> HTLPANEFRCLTPEDAAGVFEIEREAFISVSGNCPLNLDEVQHFLTLCPELSLGWFVEGRLVAFIIGSLWDEERLTQESLALHRPRGHSAHLHALAVHRSFRQQGKGSVLLWRYLHHVGAQPAVRRAVLMCEDALVPFYQRFGFHPAGPCAI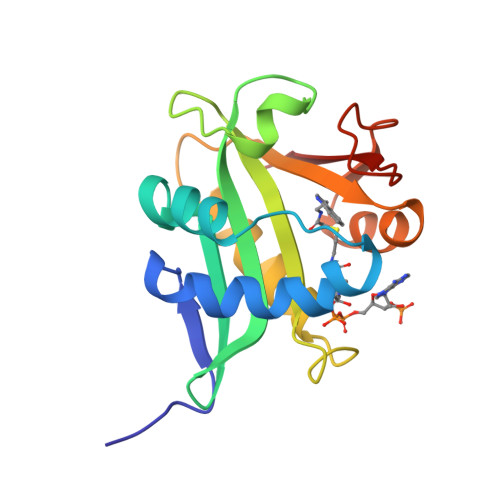VVGSLTFTEMHCSL> MKFCLYCCHCYIVICGKATHYYKSSKATSNLKSSNRVLMRNPMSPSEQHSQHNSTLAASPFVSNVSAARTQQSLPTDAQNDRLQQPWNRTNTATSPYQSLANSPLIQKLQANIMTPHQPSANSNSNSNSITGNVVNDNNLLASMSKNSMFGSTIPSTLRKVSLQREYKDSVDGVVRDEDNDEDVHNNGDAAANANNDRESKLGHNGPLTTTTLTTTTTATQLDVSELSAIERLRLWRFDALMQHMYRTAEYIADKVYNISNDPDDAFWLGQVYYNNNQYVRAVELITRNNLDGVNILCRYLLGLSFVKLQRFDDALDVIGEYNPFSEDPSTTAANTMSNNGNNSNTSQPVTDGGIKMESSLCFLRGKIYFAQNNFNKARDAFREAILVDIKNFEAFEMLLSKNLLTPQEEWDLFDSLDFKEFGEDKEIMKNLYKINLSKYINTEDITKSNEILAKDYKLADNVDVVRSKVDICYTQCKFNECLELCETVLENDEFNTNILPAYIGCLYELSNKNKLFLLSHRLAETFPKSAITWFSVATYYMSLDRISEAQKYYSKSSILDPSFAAAWLGFAHTYALEGEQDQALTAYSTASRFFPGMHLPKLFLGMQFMAMNSLNLAESY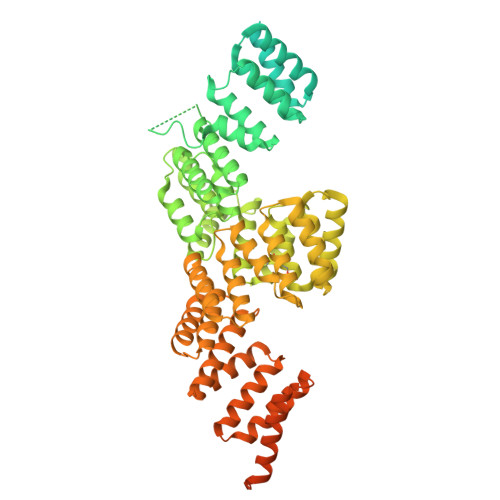FVLAYDICPNDPLVLNEMGVMYFKKNEFVKAKKYLKKALEVVKDLDPSSRTTISIQLNLGHTYRKLNENEIAIKCFRCVLEKNDKNSEIHCSLGYLYLKTKKLQKAIDHLHKSLYLKPNNSSATALLKNALELNVTLSLDASHPLIDKSNLMSQASKDKASLNKKRSSLTYDPVNMAKRLRTQKEIFDQNNKALRKGGHDSKTGSNNADDDFDADMELEKSSIPENLYF[4-(cyclopropanecarbonyl)piperazin-1-yl](furan-2-yl)methanone | C13 H16 N2 O3 | 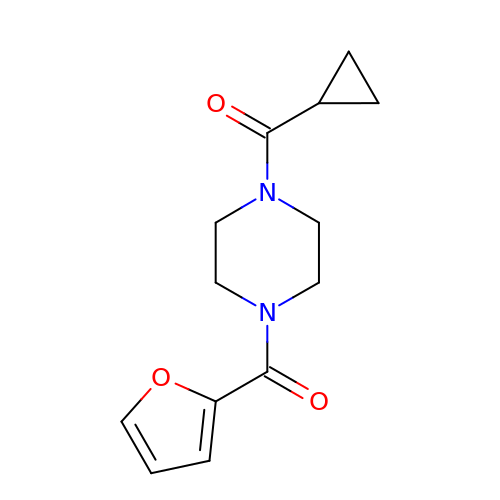SMBREKYBPARCFW-UHFFFAOYSA-N1,2-benzoxazol-3-amine | C7 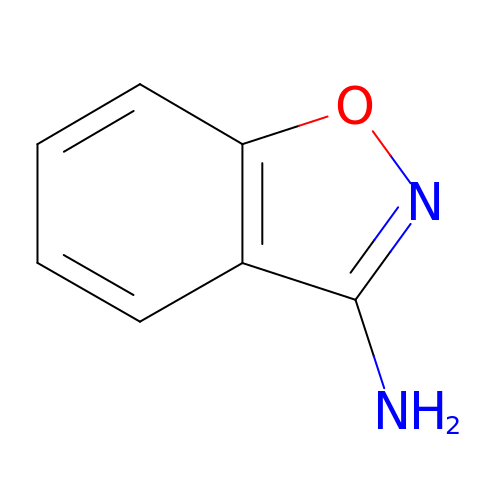H6 N2 O | NLMVYUBGWZWUGB-UHFFFAOYSA-N>[7x]SNANNLVPTVI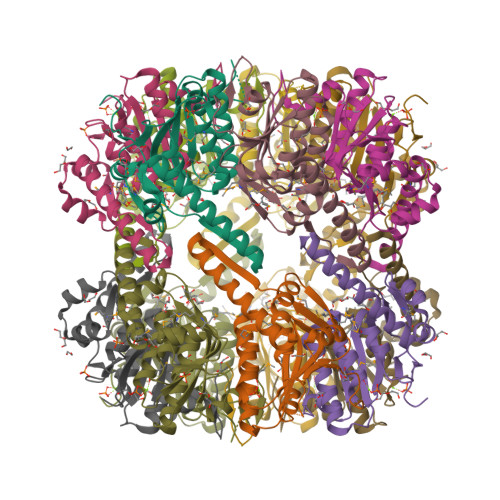EKTAGGERAFDIYSRLLKERIVFLNGEVNDHSANLVIAQLLFLESEDPDKDIYFYINSPGGMVTAGMGVYDTMQFIKPDVSTICIGLAASMGSLLLAGGAKGKRYSLPSSQIMIHQPLGGFRGQASDIEIHAKNILRIKDRLNKVLAHHTGQDLETIVKDTDRDNFMMADEAKAYGLIDHVIESREAIIK> MDQKILSLAAEKTADKLQEFLQTLREGDLTNLLQNQAVKGKVAGALLRAIFKGSPCSEEAGTLRRRKIYTCCIQLVESGDLQKEIVSEIIGLLMLEAHHFPGPLLVELANEFISAVREGSLVNGKSLELLPIILTVLATKKENLAYGKGVLSGEECKKQLINTLCSGRWDQQYVIQLTSMFKDVPLTAEEVEFVVEKALSMFSKMNLQEIPPLVYQLLVLSSKGSRKSVLEGIIAFFSALDKQHNEEQSGDELLDVVTVPSGELRHVEGTIILHIVFAIKLDYELGRELVKHLKVGQQGDSNNNLSPFSIALLLSVTRIQRFQDQVLDLLKTSVVKSFKDLQLLQGSKFLQNLVPHRSYVSTMILEVVKNSVHSWDHVTQGLVELGFILMDSYGPKKVLDGKTIETSPSLSRMPNQHACKLGANILLETFKIHEMIRQEILEQVLNRVVTRASSPISHFLDLLSNIVMYAPLVLQNCSSKVTEAFDYLSFLPLQTVQRLLKAVQPLLKVSMSMRDCLILVLRKAMFANQLDARKSAVAGFLLLLKNFKVLGSLSSSQCSQSLSVSQVHVDVHSHYNSVANETFCLEIMDSLRRCLSQQADVRLMLYEGFYDVLRRNSQLANSVMQTLLSQLKQFYEPEPDLLPPLKLEACILTQGDQISLQEPLDYLLCCIQHCLAWYKNTVIPLQQGEEEEEEEEAFYEDLDDILESITNRMIKSELEDFELDKSADFSQSTSIGIKNNISAFLVMGVCEVLIEYNFSISSFSKNRFEDILSLFMCYKKLSDILNEKAGKAKTKMANKTSDSLLSMKFVSSLLTALFRDSIQSHQESLSVLRSSNEFMRYAVNVALQKVQQLKETGHVSGPDGQNPEKIFQNLCDLTRVLLWRYTSIPTSVEESGKKEKGKSISLLCLEGLQKIFSAVQQFYQPKIQQFLRALDVTDKEGEEREDADVSVTQRTAFQIRQFQRSLLNLLSSQEEDFNSKEALLLVTVLTSLSKLLEPSSPQFVQMLSWTSKICKENSREDALFCKSLMNLLFSLHVSYKSPVILLRDLSQDIHGHLGDIDQDVEVEKTNHFAIVNLRTAAPTVCLLVLSQAEKVLEEVDWLITKLKGQVSQETLSEEASSQATLPNQPVEKAIIMQLGTLLTFFHELVQTALPSGSCVDTLLKDLCKMYTTLTALVRYYLQVCQSSGGIPKNMEKLVKLSGSHLTPLCYSFISYVQNKSKSLNYTGEKKEKPAVVATAMARVLRETKPIPNLIFAIEQYEKFLIHLSKKSKVSLMQHMKLSTSRDFKIKGNILDMVLREDGEDENEEGTASEHGGQNKEPAKKKRKK;> MVSKRRLSKSEDKESLTEDASKTRKQPLSKKTKKSHIANEVEENDSIFVKLLKISGIILKTGESQNQLAVDQIAFQKKLFQTLRRHPSYPKIIEEFVSGLESYIEDEDSFRNCLLSCERLQDEEASMGASYSKSLIKLLLGIDILQPAIIKTLFEKLPEYFFENKNSDEINIPRLIVSQLKWLDRVVDGKDLTTKIMQLISIAPENLQHDIITSLPEILGDSQHADVGKELSDLLIENTSLTVPILDVLSSLRLDPNFLLKVRQLVMDKLSSIRLEDLPVIIKFILHSVTAMDTLEVISELREKLDLQHCVLPSRLQASQVKLKSKGRASSSGNQESSGQSCIILLFDVIKSAIRYEKTISEAWIKAIENTASVSEHKVFDLVMLFIIYSTNTQTKKYIDRVLRNKIRSGCIQEQLLQSTFSVHYLVLKDMCSSILSLAQSLLHSLDQSIISFGSLLYKYAFKFFDTYCQQEVVGALVTHICSGNEAEVDTALDVLLELVVLNPSAMMMNAVFVKGILDYLDNISPQQIRKLFYVLSTLAFSKQNEASSHIQDDMHLVIRKQLSSTVFKYKLIGIIGAVTMAGIMAADRSESPSLTQERANLSDEQCTQVTSLLQLVHSCSEQSPQASALYYDEFANLIQHEKLDPKALEWVGQTICNDFQDAFVVDSCVVPEGDFPFPVKALYGLEEYDTQNGIAINLLPLLFSQDFAKDGGPVTSQESGQKLVSPLCLAPYFRLLRLCVERQHNGNLEEIDGLLDCPIFLTDLEPGEKLESMSAKERSFMCSLIFLTLNWFREIVNAFCQETSPEMKGKVLTRLKHIVELQIILEKYLAVTPDYVPPLGNFDVETLDITPHTVTAISAKIRKKGKIERKQKTDGSKTSSSDTLSEEKNSECDPTPSHRGQLNKEFTGKEEKTSLLLHNSHAFFRELDIEVFSILHCGLVTKFILDTEMHTEATEVVQLGPPELLFLLEDLSQKLESMLTPPIARRVPFLKNKGSRNIGFSHLQQRSAQEIVHCVFQLLTPMCNHLENIHNYFQCLAAENHGVVDGPGVKVQEYHIMSSCYQRLLQIFHGLFAWSGFSQPENQNLLYSALHVLSSRLKQGEHSQPLEELLSQSVHYLQNFHQSIPSFQCALYLIRLLMVILEKSTASAQNKEKIASLARQFLCRVWPSGDKEKSNISNDQLHALLCIYLEHTESILKAIEEIAGVGVPELINSPKDA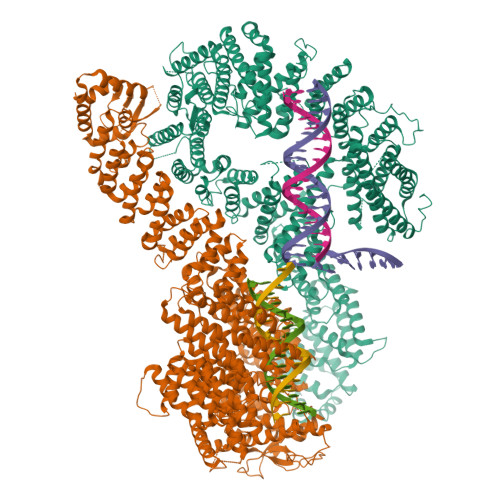SSSTFPTLTRHTFVVFFRVMMAELEKTVKKIEPGTAADSQQIHEEKLLYWNMAVRDFSILINLIKVFDSHPVLHVCLKYGRLFVEAFLKQCMPLLDFSFRKHREDVLSLLETFQLDTRLLHHLCGHSKIHQDTRLTQHVPLLKKTLELLVCRVKAMLTLNNCREAFWLGNLKNRDLQGEEIKSQNSQESTADESEDDMSSQASKSKATEDGEEDEVSAGEKEQDSDESYDDSD>GPGSELPQMVQQLNSPDQQELQSALRKLQQIAMGGNEQIQAVIDAGALPALVQLLSSPNEQILASALGALANIASGGNEQIQAVIDAGALPALVQLLSSPNEQILQFALIALANIASGGNEQIQAVIDAGALPALVQLLSSPNEQILQEALWALSNIASGGNEQIQAVIDAGALPALVQLLSSPNEQILQEALWALSN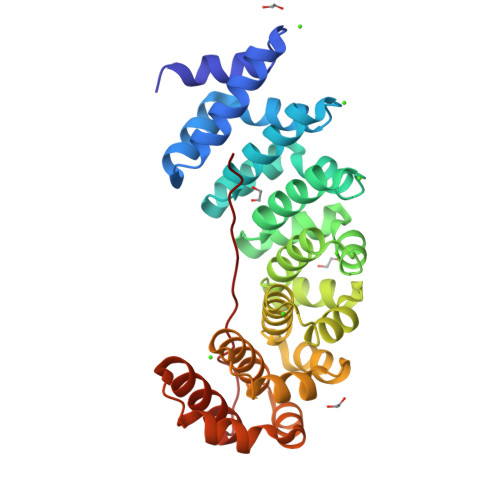IASGGNEQIQAVIDAGALPALVQLLSSPNEQILQEALWALSNIASGGNEQKQAVKEAGALEKLEQLQSHENEKIQKEAQEALEKLQSHGSGGSGKRKRKAKITW[6x]>SNAEELIEIREARMDDLDTIAKFNYNLAKETEGKELDMDVLTKGVKALLLDERKGKYHVYTVFDKVVAQIMYTYEWSDWRNGNFLWIQSVYVDKEYRRKGIFNYLFNYIKNICDKDENIVGMRLYVEKENINAKATYESLNMYECDYNMYEYEVIHS[2x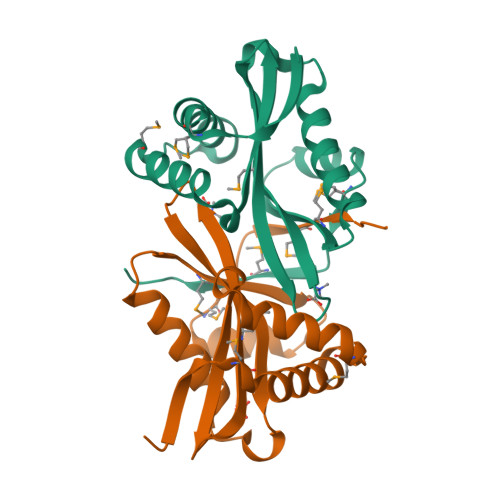]(5~{S})-7-[[2,6-bis(fluoranyl)phenyl]methyl]-3-(3-methylthiophen-2-yl)-1-oxa-2,7-diazaspiro[4.4]non-2-en-6-one 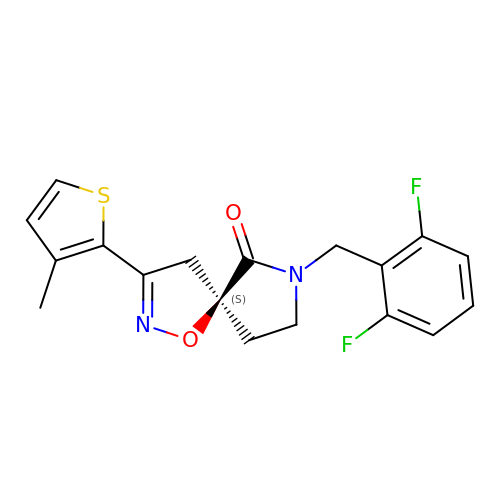| C18 H16 F2 N2 O2 S | LDAZTXWVKWXAJU-SFHVURJKSA-N> VGSLNCIVAVSQNMGIGKNGDLPWPPLRNEFRYFSRMTTTSSVEGKQNLVIMGKKTWFSIPEKFRPLKGRINLVLSRELKEP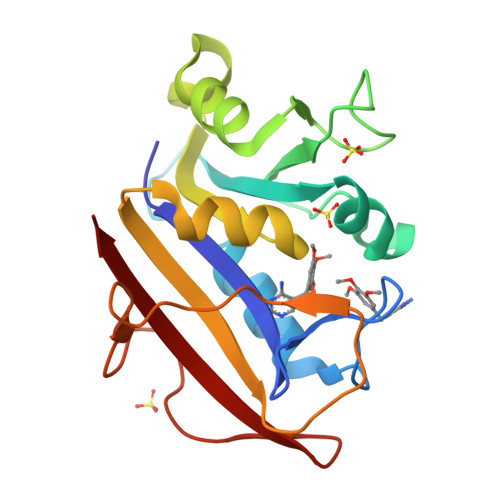PQGAHFLSRSLDDALKLTEQPELANKVDMVWIVGGSSVYKEAMNHPGHLKLFVTRIMQDFESDTFFPEIDLEKYKLLPEYPGVLSDVQEEKGIKYKFEVYEKND> MNYNLSKYPDDVSRLFKPRPPLSYKRPTDYPYAKRQTNPNITGVANLLSTSLKHYMEEFPEGSPNNHLQRYEDIKLSKIKNAQLLDRRLQNWNPNVDPHIKDTDPYRTIFIGRLPYDLDEIELQKYFVKFGEIEKIRIVKDKITQKSKGYAFIVFKDPISSKMAFKEIGVHRGIQIKDRICIVDIERGRTVKYFKPRRLGGGLGGRGYSNRDSRLPGRFASASTSNPAERNYAPRLPRRETSSSAYSADRYGSSTLDARYRGNRPLLSAATPTAAVTSVYKSRNSRTRESQPAPKEAPDY;> MTRYYCEYCHSYLTHDTLSVRKSHLVGKNHLRITADYYRNKARDIINKHNHKRRHIGKRGRKERENSSQNETLKVTCLSNKEKRHIMHVKKMNQKELAQTSIDTLKLLYDGSPGYSKVFVDANRFDIGDLVKASKLPQRANEKSAHHSFKQTSRSRDETCESNPFPRLNNPKKLEPPKILSQWSNTIPKTSIFYSVDILQTTIKESKKRMHSDGIRKPSSANGYKRRRYGN;> MSALYFQNLPSRPANKENYTRLLLKHINPNNKYAINPSLPLPHNKLQISSQPLMLLDDQMGLLEVSISRSSKMTNQAFLTFVTQEEADRFLEKYTTTALKVQGRKVRMGKARTNSLLGLSIEMQKKKGNDETYNLDIKKVLKARKLKRKLRSDDICAKKFRLKRQIRRLKHKLRSRKVEEAEIDRIVKEFETRRLENMKSQQENLKQSQKPLKRAKVSNTMENPPNKVLLIQNLPSGTTEQLLSQILGNEALVEIRLVSVRNLAFVEYETVADATKIKNQLGSTYKLQNNDVTIGFAKGRRIPGLINPWKRRWKKNFIAVSAANRFKKISSSGALDYDIPTTASENLYFQ;> MDKYTALIHDENFSTLTLNVSRYPKSLAYWEKLLNYIVKASAPICKSTEPQLLKLIRCTYSSMLNEFPYLENYYIDFALLEYKLGNVSMSHKIFQRGLQAFNQRSLLLWTSYLKFCNNVISHQKQLFKKYETAEEYVGLHFFSGEFWDLYLEQISSRCTSSKKYWNVLRKILEIPLHSFSKFYALWLQRIDDIMDLKQLSQLTSKDELLKKLKIDINYSGRKGPYLQDAKKKLKKITKEMYMVVQYQVLEIYSIFESKIYINYYTSPETLVSSDEIETWIKYLDYTITLQTDSLTHLNFQRALLPLAHYDLVWIKYSKWLINSKNDLLGAKNVLLMGLKFSLKKTEIIKLLYSVICKLNEYVLLRNLLEKIESSYSDNVENVDDFEIFWDYLQFKTFCQNSLYSSRYSDSQSNGLLNKELFDKVWKRLSCKEKKSGQEILLNNLVQFYSKDTVEFVEKNIFQKIIEFGWEYYLQNGMFWNCYCRLIYFDTSRSYLDKRQYIVRKIWPQIDKKFAQSVLPSLTEFCESYFPEEMDTLEEMFTEEP;> MPDETNFTIEDIEPRPDALRGLDTQFLQDNTALVQAYRGLDWSDISSLTQMVDVIEQTVVKYGNPNDSIKLALETILWQILRKYPLLFGFWKRFATIEYQLFGLKKSIAVLATSVKWFPTSLELWCDYLNVLCVNNPNETDFIRNNFEIAKDLIGKQFLSHPFWDKFIEFEVGQKNWHNVQRIYEYIIEVPLHQYARFFTSYKKFLNEKNLKTTRNIDIVLRKTQTTVNEIWQFESKIKQPFFNLGQVLNDDLENWSRYLKFVTDPSKSLDKEFVMSVFDRCLIPCLYHENTWMMYIKWLTKKNISDEVVVDIYQKANTFLPLDFKTLRYDFLRFLKRKYRSNNTLFNNIFNETVSRYLKIWPNDILLMTEYLCMLKRHSFKNSLDQSPKEILEKQTSFTKILETSITNYINNQIDAKVHLQTLINDKNLSIVVVELIKTTWLVLKNNMQTRKYFNLYQKNILIKNSVPFWLTYYKFEKSNVNFTKLNKFIRELGVEIYLPTTVMNDILTDYKTFYLTHSNIVTYESSIIDSNTFDPILYPELKMSNPKYDPVLNTTANVDWHKKTEWKEAGHIGITTERPQISNSIIECNSGTLIQKPISLPNFRNLEKINQVKINDLYTEEFLKEGK;> MSYKQTTYYPSRGNLVRNDSSPYTNTISSETNNSSTSVLSLQGASNVSLGTTGNQLYMGDLDPTWDKNTVRQIWASLGEANINVRMMWNNTLNNGSRSSMGPKNNQGYCFVDFPSSTHAANALLKNGMLIPNFPNKKLKLNWATSSYSNSNNSLNNVKSGNNCSIFVGDLAPNVTESQLFELFINRYASTSHAKIVHDQVTGMSKGYGFVKFTNSDEQQLALSEMQGVFLNGRAIKVGPTSGQQQHVSGNNDYNRSSSSLNNENVDSRFLSKGQSFLSNGNNNMGFKRNHMSQFIYPVQQQPSLNHFTDPNNTTVFIGGLSSLVTEDELRAYFQPFGTIVYVKIPVGKCCGFVQYVDRLSAEAAIAGMQGFPIANSRVRLSWGRSAKQTALLQQAMLSNSLQVQQQQPGLQQPNYGYIPSSTCEAPVLPDNNVSSTMLPGCQILNYSNPYANANGLGSNNFSFYSNNNATNTQATSLLADTSSMDLSGTGGQQVIMQGSEAVVNSTNAMLNRLEQGSNGFMFA;> MRPRRRGLAYHHTKPKGQLSQGHYPTTSNDGQRRKVGNSEAFQSFDIWKNLDRIRSTKKNAGQFIKGSLLILPMRTEDKQQFDECMDELHKYISKDILRCYPQKEQKDEGMLFYIVLKDFNILDSCFVLSVLLAFQKRLWMAPSEKSYFRVPKNINLTGSFYLPKNIETGRGHIITSYRREQPSSSIVEVGFNVVPDFQQFQVKACHVSKFMNELSNFFSQVEFGKCEANVINYFKREYNRTYSQISLALYELPLIGDGLFDIKSYISKTRPIIETSKAQMIKHISEMKAYNEISGLQGDQFPRQQRPLSNSPSSNSISSSQTIEAGATSYQTQPQRHAVNKPSNVLNSSNRHSGPKTFEDGRYSEGNKPGFMTQDEIKQHCIGTIKASMDAVKKKSSYQILKTYVRCPRQNYIDIVYQNLNDLRSKTNCNIVVLNLNNLHESQMWLESLNTTNYTIFAQAPHPSTIRVISIGGVGEYIVKALELILNILEH;> MSTMSTPAAEQRKLVEQLMGRDFSFRHNRYSHQKRDLGLHDPKICKSYLVGECPYDLFQGTKQSLGKCPQMHLTKHKIQYEREVKQGKTFPEFEREYLAILSRFVNECNGQISVALQNLKHTAEERMKIQQVTEELDVLDVRIGLMGQEIDSLIRADEVSMGMLQSVKLQELISKRKEVAKRVRNITENVGQSAQQKLQVCEVCGAYLSRLDTDRRL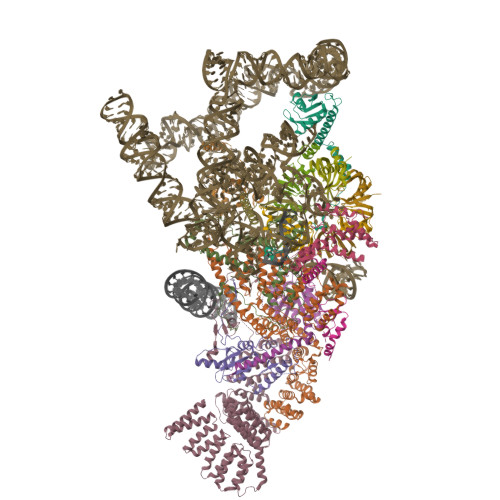ADHFLGKIHLGYVKMREDYDRLMKNNRTTNASKTATTLPGRRFV;> MSKIQVAHSSRLANLIDYKLRVLTQDGRVYIGQLMAFDKHMNLVLNECIEERVPKTQLDKLRPRKDSKDGTTLNIKVEKRVLGLTILRGEQILSTVVEDKPLLSKKERLVRDKKEKKQAQKQTKLRKEKEKKPGKIAKPNTANAKHTSSNSREIAQPSSSRYNGGNDNIGANRSRFNNEAPPQTRKFQPPPGFKRK;> MKLVNFLKKLRNEQVTIELKNGTTVWGTLQSVSPQMNAILTDVKLTLPQPRLNKLNSNGIAMASLYLTGGQQPTASDNIASLQYINIRGNTIRQIILPDSLNLDSLLVDQKQLNSLRRSGQIANDPSKKRRRDFGAPANKRPRRGL;> MSSQIIDRPKHELSRAELEELEEFEFKHGPMSLINDAMVTRTPVIISLRNNHKIIARVKAFDRHCNMVLENVKELWTEKKGKNVINRERFISKLFLRGDSVIVVLKTPVE;> MTMNGIPVKLLNEAQGHIVSLELTTGATYRGKLVESEDSMNVQLRDVIATEPQGAVTHMDQIFVRGSQIKFIVVPDLLKNAPLFKKNSSRPMPPIRGPKRR;> MSNKVKTKAMVPPINCIFNFLQQQTPVTIWLFEQIGIRIKGKIVGFDEFMNVVIDEAVEIPVNSADGKEDVEKGTPLGKILLKGDNITLITSAD;> MSESSDISAMQPVNPKPFLKGLVNHRVGVKLKFNSTEYRGTLVSTDNYFNLQLNEAEEFVAGVSHGTLGEIFIRCNNVLYIRELPN;> MVSTPELKKYMDKKILLNINGSRKVAGILRGYDIFLNVVLDDAMEINGEDPANNHQLGLQTVIRGNSIISLEALDAI>AHQPVPQFPDRHEIFDVNAIRADFPILRETVNGKPLIWFDNAATTQKPQAVIDRLSHFYAHENSNIHRAAHELAARATDAYEDAREAVRRFIGAAKAEEIIFLRGTTEAINLVAHAWGGKHLGPGDEIVITHLEHHANIVPWQLLSRQTGAVLKVAPVDDAGNLLLGEFEDLLGPRTKLVAATQVSNALGTVTPVETIVELGHRYGARVLIDGAQSIPHMPIDVAALGADFFVFSGHKIYGPTGIGVLYGREDALAETPPWQGGGNMIADVTLERSLYQGPPNKFEAGTGNIADAVGLGEAIRYVERVGIERIAAYEHALLEYATPRLAAIPGVRIVGTAQEKASVLSFVLAGHEPLEVGK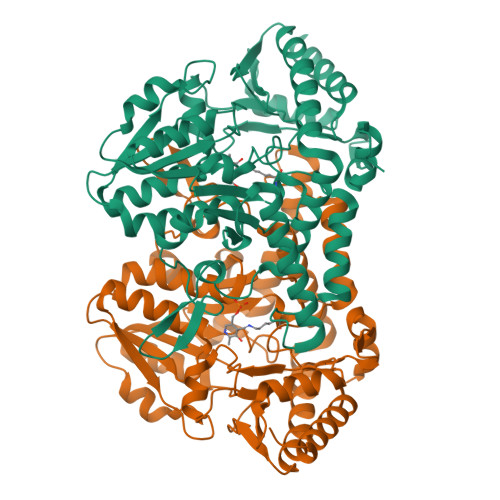ALNAEGIAVRAGHHCAQPILRRMGLEATVRPSFAFYNTFDEIDVFIDAVRRIAEGSVDYKDDDDK[2x]(2S)-2-azanyl-6-(trimethylsilylmethoxycarbonylamino)hexanoic acid | C11 H24 N2 O4 Si 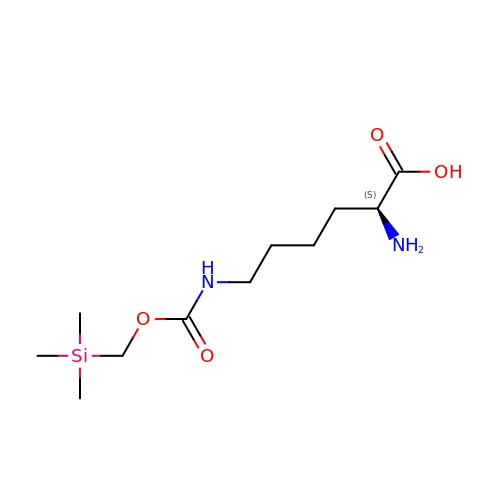| WFRSGOQCYVJZDV-VIFPVBQESA-N> AANSVVAYGRWPEYLRDSEANPVDQPTEPDVAACRFYTLDTVSWTKESRGWWWKLPDALRDMGLFGQNMYYHYLGRSGYTVHVQCNASKFHQGALGVFAVPEMCLAGDSNTTTMHTSYQNANPGEKGGTFTGTFTPDNNQ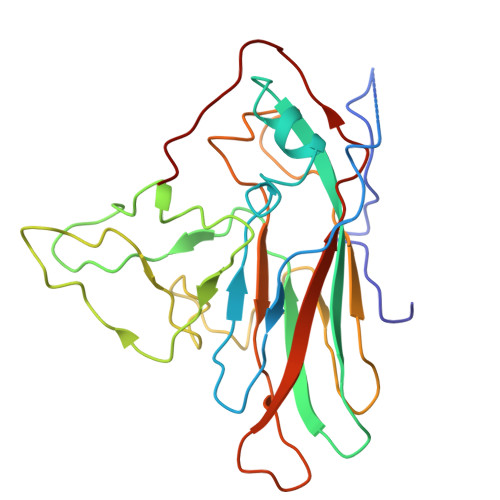TSPARRFCPVDYLLGNGTLLGNAFVFPHQIINLRTNNCATLVLPYVNSLSIDSMVKHNNWGIAILPLAPLNFASESSPEIPITLTIAPMCCEFNGLRNITLPRLQ>[6x]MGGEVEEPEPQMVLSPLTSAAIFLVVTIDSGGEDTVRDLLSDVASLERAVGFRAQPDGRLSCVTGIGSEAWDRLFSGARPAGLHPFRELDGPVHRAVATPGDLLFHIRASRLDLCFALATEIMGRLRGAVTPQDEVHGFKYFDERDMLGFVDGTENPTGAAARRAVLVGAEDPAFAGGSYAVVQKYLHDIDAWEGLSVEAQERVIGRRKMTDVELSDDVKPADSHVALTSVTGPDGSDLEILRDNMPFGSVGREEFGTYFIGYARTPEVTETMLERMFLGTASAPHDRILDFSTAVTGSLFFTPAADFLEDLSARP

Dye‐decolorising peroxidases (DyPs) are the most recent member of the peroxidase family to be discovered. Three DyPs have been identified in S. lividans; two A‐types (DtpA and DtpAa) and one B‐type (DtpB). Using serial femtosecond X‐ray crystallography (SFX), we have determined the pristine structures of the FeIII and FeIV=O redox states of a B‐type DyP. These structures reveal a water‐free distal heme site that, together with the presence of an asparagine, imply the use of the distal arginine as a catalytic base.

To seek further structural confirmation for a “dry” distal site in FeIII‐DtpB a composite X‐ray structure of FeIII‐DtpB at 100 K was determined. Consistent with the SFX structure, the spectroscopically‐validated 100 K composite structure also revealed a penta‐coordinate and out of plane heme‐Fe and importantly confirmed the absence of a H2O‐Asp unit. The heme redox state in the crystals was corroborated through analysis of larger DtpB crystals suitable to obtain electronic absorbance spectra at 100 K. Identical electronic absorbance bands to those for FeIII‐DtpB and compound I in solution were observed in the crystals. The heme‐Fe in DtpB is penta‐coordinate and sits out of the porphyrin plane towards the proximal His225 ligand. The distal heme site in the immediate vicinity of the Asp/Arg couple of FeIII‐DtpB is thus “dry”, which has the effect of isolating Asp152 from communication with the heme. The absence of a distal heme‐Fe H2O chain in FeIII‐DtpB coincides with the protrusion into the distal site of Asn245, with its side chain amide occupying the spatial position where a H2O molecule (w2) is located and H‐bonded to the distal Asp in the FeIII‐DtpA and FeIII‐DtpAa structures.> MKLSKDTTALLKNFATINSGIMLKSGQFIMTRAVNGTTYAEANISDVIDFDVAIYDLNGFLGILSLVNDDAEISQSEDGNIKIADARSTIFWPAADPSTVVAPNKPIPFPVASAVTEIKAEDLQQLLRVSRGLQIDTIAITVKEGKIVINGFNKVEDSALTRV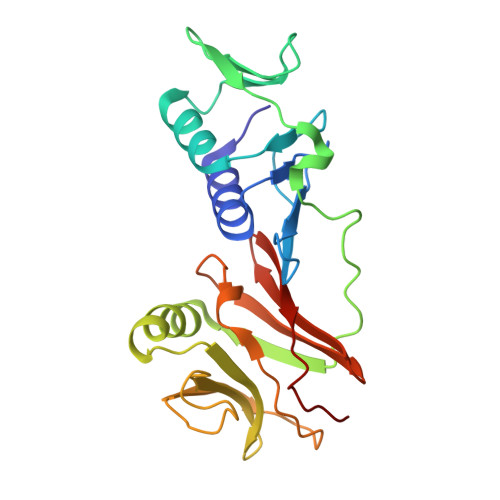KYSLTLGDYDGENTFNFIINMANMKMQPGNYKLLLWAKGKQGAAKFEGEHANYVVALEADSTHDF> KILHR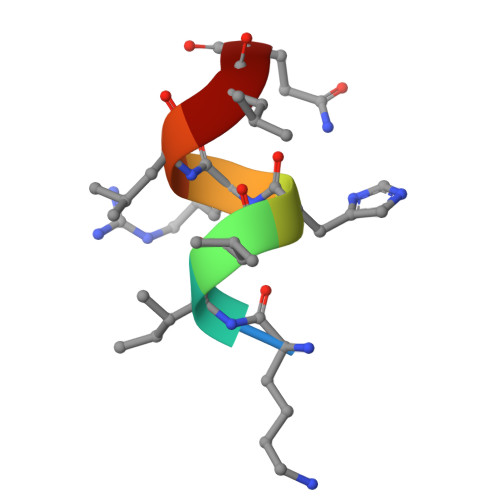LLQ> MEGLNLVATALAVGLGAIGPGVGIGIIVSGAVQAIGRNPEIENRVVTYMFI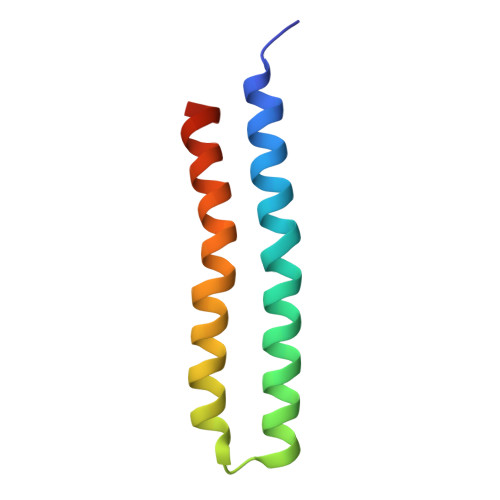GIAFTEALAIFGLVIAFLIGFGVLQ>ASGQATERALGRRTIPAGEARSIIIRQRYDAPVDEVWSACTDPNRINRWFIEPKGDLREGGNFALQGNASGDILRCEPPRRLTISWVYEGKPDSEVELRLSEEGDGTLLELEHATTSEQMLVEVGVGWEMALDFLGMFIRGDLPGGPVPEDA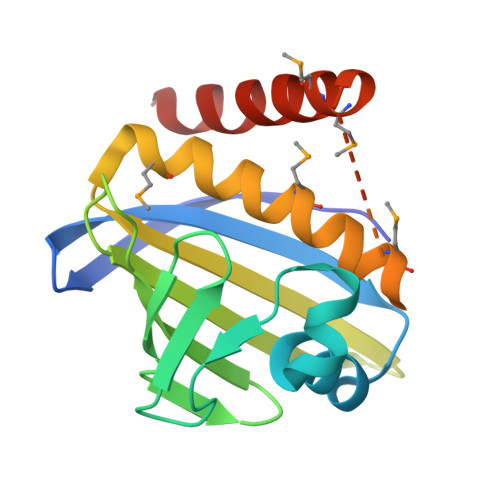AEEFEPSPEMMRISQERGEAWAALVHSGS[2x]>MAHHHHHHSSGLEVLFQGPMIEIPSAATASPQYPQRRACPYRPAGGYERPVTRVRLYDGRPAWLVTGHETARQVLLDAATFSSDRQHPAFPALAARFEAARAVRNFIGMDPPEHTAQRRMLISGFTAKRVATLRPAITEIVDSLLDEVVRRGPGVDLVATFTLPVPSVVICRLLGVPYADHEFFEH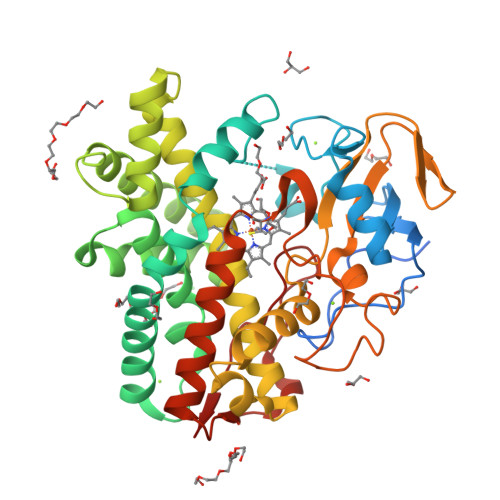QSRRIAAGTSTAAESADAFGQLKRYLLGLIETKGRGGEDMLDVLVDEQVATGTVTTPDLVDLALLLLVAGHETTASTLALGVALLLEQDGGAVAADPTRVGAVVEEILRHTAVADGVARFATRDTEVAGVRIAAGDAVVVALSAANRDPGPFPDPDRFDPRRGGRQHVTFGHGPHQCIGANLARAELEIALSRLFTRLPTLALAVPVEELGGKEAGGVQGVQRLPVTW[2x]>EPEEVIPSRLDIRVGKIITVEKHPDADSLYVEKIDVGEAEPRTVVSGLVQFVPKEELQDRLVVVLCNL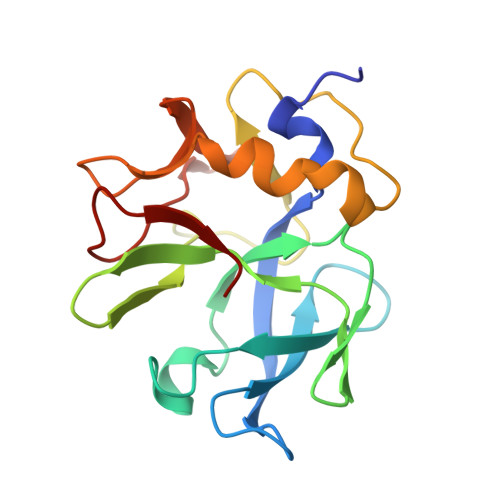KPQKMRGVESQGMLLCASIEGINRQVEPLDPPAGSAPGEHVFVKGYEKGQPDEELKPKKKVFEKLQADFKISEECIAQWKQTNFMTKLGSISCKSLKGGNISLE[4x]>GDDGNYCKRTPLYIDFKEIGWDSWIIAPPGYEAYECRGVCFFPLAEHLTPTKHAIIQTLVHLKNSQKASKACCVPTKLEPISILYLDKGVVTLKYKYEGMAVSECGCR[2x]

BMP-9 and BMP-10 are TGF-β family signaling ligands naturally secreted into blood. They act on endothelial cells and are required for proper development and maintenance of the vasculature. BMP-9 and −10 are synthesized as pro-proteins and processed by furin to release growth factors comprised of two cystine-knotted protomers that can covalently homo- or hetero-dimerize via a single cysteine in the dimer interface. Unlike other ligands of the TGF-β family, BMP-9 and −10 are secreted as a mixture of disulfide-linked dimers and monomers, in which the interchain cysteine (Cys-392) remains either paired or unpaired.

Attempts were made to crystallize BMP-10 and obtain a high-resolution structure. While BMP-10 crystallized in many conditions, none of these crystals diffracted to high resolution. A chimeric BMP-10 with five surface residues replaced with BMP-9 crystal contacts (N357F, Y358F, A374T, Y409L, F411Y) was purified, crystallized, and solved. Unfortunately, the condition was at pH 6.2 and the crystal contacts disrupted the residues adjacent to the interchain disulfide, thus neither strain nor radiation sensitivity were observed in the chimeric BMP-10. Crystals of the BMP-10 Crystal Chimera formed at room temperature in a one-to-one mixture of 5.0 mg mL−1 protein and 25%(v/v) 1,2-propanediol, 100 mM sodium phosphate dibasic/potassium phosphate monobasic pH 6.2, 10% (v/v) glycerol (Rigaku Wizard Cryos E11). Unfortunately, an analogous analysis could not be performed on any BMP-10 structure due to both limited resolution and local disruptions (caused by pH, type-l receptors, or crystal contacts) in BMP-10 crystals. As such, the extended analyses of BMP-10 are limited to disulfide bonded cysteines in published structures, and it is not clear whether differences in these structures are due to deformations caused by local disruptions or fundamental differences in BMP-10.The crystallographic analysis of a lipase from Palaeococcus ferrophilus (PFL) previously annotated as a lysophospholipase revealed high structural conservation with other monoglyceride lipases, in particular in the lid domain and substrate binding pockets. In agreement with this observation, PFL was shown to be active on various monoacylglycerols. Many lipases have evolved to contain a so-called cap domain, which, in MGLs, consists in an insertion after the β6 sheet of the α/β hydrolase core domain and participates in the substrate recognition or serves as a lid to control the access to the active site. The ligand binding pocket is lined by well-conserved residues, which explains the PFL substrate preference for monoacylglycerols compared to other lipids, particularly lysophospholipids.

Despite a limited sequence identity with hMGL or mtMGL, PFL displays a high level of structural conservation with these enzymes. The proposed glycerol exit route is locked by Leu144, which corresponds to the gatekeeper residue Ile179 in hMGL and lies in an intermediate state between the open and closed states of the human enzyme. A comparison of the van der Waals surface of the crystal structure of PFL, and a closed structure observed for the PFL-G system, allows emphasizing the partial opening of the crystal structure (respectively). Figure S5A also reports that the lid of the crystal structure of PFL is seen as partially open when a spherical probe with a radius size of up to 2.1 Å only is used, while the residues Leu144 and His166 delineate a very small aperture toward the alcohol-binding pocket that is not accessible to the solvent. The H5 helix, which constitutes the core of the cap, its hinges, but also the H7 and H8 helices, located at the close vicinity, are the most flexible parts of the enzyme. Nevertheless, micellar concentrations of LDAO impede the association of the dimer toward higher oligomeric forms and allow the crystallization of the enzyme. Indeed, crystals of PFL could not be obtained in the absence of LDAO or, on the contrary, in the presence of MAFP, which suggests that this inhibitor stabilizes an alternate conformation compared to the crystal form. Particularly, the Ser117–Ile204 hydrogen bond is observed in the presence of the LDAO ligand, and Asn142 can play a closure function even at high temperature. In the present study, we highlight Phe123 as a residue is involved in the closure of the PFL lid, which mirrors the corresponding pulling residue identified earlier for the hMGL. The high flexibility and closure propensity of the lid observed in the MD study, even in the presence of LDAO, could constitute indications that the crystal packing contributes at least in part to the stabilization of the conformational state highlighted in the experimental structure.

>[2x]MELYRAKFGTPERGWVVLVHGLGEHSGRYGKLIELLNGAGFGVYAFDWPGHGKSPGKRGHTSVEEAMKIIDSIIEELGEKPFLFGHSLGGLTVIRYAETRPDKIMGVVASSPALAKSPKTPSFMVALAKVLGRITPGLSLSNGLDPKLLSRNPDAVKRYIEDPLVHDRISGKLGMSVFDNMERAHKEAERIKAPVLLLVGTADIITPPEGSRRLFEELKVKDKTIMEFKGAYHEIFEDPEWGEEFHRAIVEWLVSHSRGDLEWASAERASSIMGDSAHHHHHH>PKFFYIK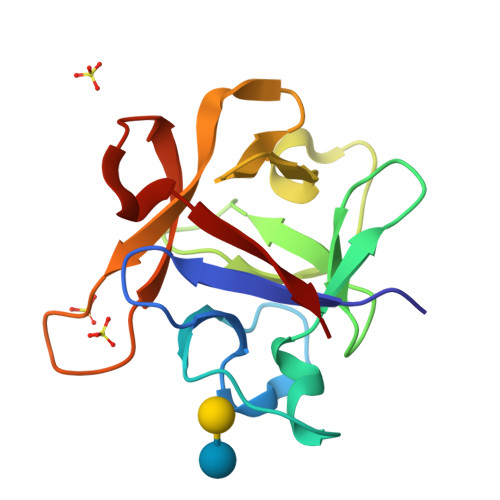SELNGKVLDIGGQNPAPGSKIITWDQKKGPTAVNQLWYTDQQGVIRSKLNDFAIDASHEQIETQPFDPNNPKRAWIVSGNTIAQLSDRDNVLGVIKSDKGASAHICAWKQHGGPNQKFIIESE[2x]> GPLGSLCGRVFKVGEPTYSCRDCAVDPTCVLCMECFLGSIHRDHRYRMTTSG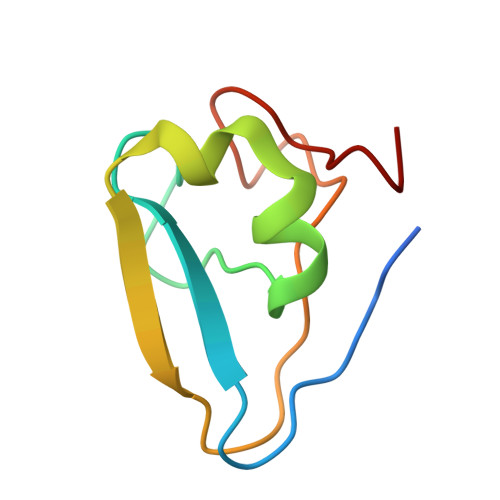GGGFCDCGDTEAWKEGPYCQKHE HAMP domains are small modules, approximately 50 amino acids, that dimerize to form an entirely parallel four-helix bundle with two helices (AS1 and AS2) supplied from each subunit. A semi-structured connector separates the AS1 and AS2 helices and contains two conserved hydrophobic residues, termed HR1 and HR2. Aer2 is a soluble receptor that contains three N-terminal HAMP domains, a gas-sensing, heme-containing PAS domain, two additional HAMP domains, and an MCP KCM. The three N-terminal HAMP domains of Aer2 (named HAMP1, HAMP2, and HAMP3 from N- to C-terminus) provide examples of two distinctly different conformations: HAMP1 and HAMP3 are similar to the Af1503 NMR structure, whereas HAMP2 has a comparatively distorted four-helix bundle structure in which the AS2 helices approximate a two-helix coiled coil and the AS1 helices splay outward at the C-terminal end.

Crystals of L44H and V33G proteins were obtained in the context of Aer2 1–172 using conditions similar to those of the native protein. V33G crystallized in the same space group as WT, but L44H produced a different crystal lattice. The V33G mutation locally destabilized the connector around HR2 and increased mobility in this region of the protein, as evidenced by decreased electron density of the connector in the region of T31–V33. These changes had no effect on the helical positions of AS1 and AS2 compared to the WT structure, which is consistent with a HAMP1 conformer generating CW output. However, the increased flexibility of the connector and loss of the V33 side chain for packing into the bundle core should affect the ability of HR2 to stabilize the HAMP2 structure, and thus we expected this substitution to disfavor conversion to a HAMP2-like conformer. Compared to H1, H1 V33G had increased CW bias in CheRB+ cells and was also CW locked in CheRB− cells. Temporal assays confirmed an inverse Asp response by H1 V33G, in that Asp caused a drastic switch from 16% to 100% CW bias. The mechanism underlying H1 V33G inverted signaling is not completely understood; however, it is clear that a branched hydrophobic residue at HR2 is important to achieve the HAMP2 conformation and CCW signaling state. Thus, it is perhaps reasonable that upon attractant binding, the V33G variant is unable to switch to a HAMP2 conformation. Stabilization of a HAMP1 state by V33G is evident by the effect of this mutation in the CheRB− background, where it produces an exclusively CW state.

> GSHMGLFNAHAVAQQRADRIATLLQSFADGQLDTAGGEAPAPGYERLYDSLRALQRQLREQRAELQQVESLEAGLAEMSRQHEAGWIDQTIPAERLEGRAARIAKGVNELVAAHIAVKMKVVSVVTAYGQGNFEPLMDRLPGKKAQITEAIDGVRERLRGAAEATSAQLATAAYN5'-O-[(S)-{[(S)-[(3R)-4-({(1E)-3-[(2-{[(2S)-2-carboxybutanoyl]sulfanyl}ethyl)amino]-3-oxoprop-1-en-1-yl}amino)-3-hydroxy-2,2-dimethyl-4-oxobutoxy](hydroxy)phosphoryl]oxy}(hydroxy)phosphoryl]adenosine 3'-(dihydrogen phosphate) | C26 H40 N7 O19 P3 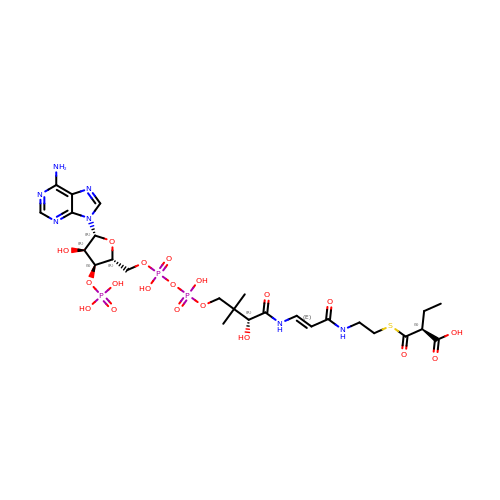S | FBYIVOIRCUIQPJ-YWIQEZFGSA-N>IEPENIGPTFSALPPIYIPTG[6x];>MHHHHHHTLPAFGFAFNASAPQFASLFTPLLLPSVSPNPNIPVPVINDTVSVGDGIRILRAGIYQISYTLTIS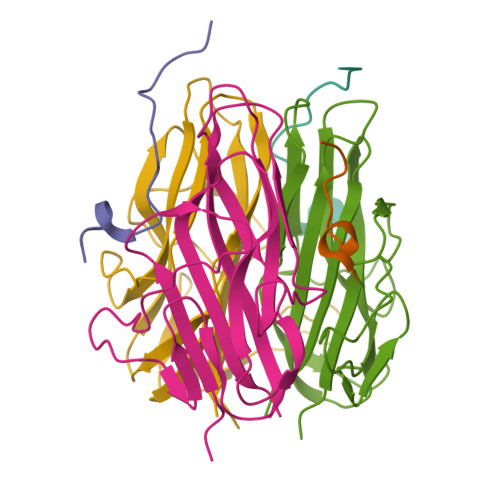LDNSPVAPEAGRFFLSLGTPANIIPGSGTAVRSNVIGTGEVDVSSGVILINLNPGDLIQIVPVQLIGTVDIRAAALTVAQIS[6x]Recently, we characterized TgCyp23 among the various Cyps of the parasite, demonstrating its high PPIase activity and its ability to bind cyclosporin A (CsA), a well‐known inhibitor of Cyps (Favretto et al., 2023). TgCyp23 exhibits the typical eight‐stranded antiparallel β‐barrel structure, with two α‐helices flanking the barrel on either side, all of them connected by loops. TgCyp23 shows remarkable sequence identity with human CypA (~52% of identity) but has a 40‐aminoacid N‐terminal extension. Here, three new structures of the protein in complex with the three non‐immunosuppressive derivatives NIM811, dhCsA, and Alisporivir have been solved at 1.17, 1.20, and 1.20 Å resolution, respectively.

Dihydrocyclosporin A (dhCsA), a closely related co‐metabolite of CsA, presents a saturation of the double bond of the unusual amino acid (4R)‐4‐([E]‐2‐butenyl)‐4‐methyl‐N‐methyl‐(L)‐threonine (MeBmt‐1) in position 1, has minimal reported immunosuppressive activity, and serves as a control in determining the role of immunosuppression in CsA‐based treatment of parasitic infections (Chappell et al., 1987; Meier et al., 1990). CsA derivatives with modifications at residue 1 (such as dhCsA, which is a co‐metabolite of CsA used as a control to determine the role of CsA in pharmacology) have also shown decreased immunosuppressive activity without compromising Cyp affinity, even though the MeBmt‐1 side chain is positioned in the part of CsA involved in the binding of Cyp (Aebi et al., 1990; Mikol et al., 1993; Rich et al., 1989). NIM811, dhCsA, and Alisporivir are attached to the CsA binding pocket. The backbone for these three derivatives is nearly identical to that of CsA. Remarkably, all the modifications in the non‐immunosuppressive derivatives are exposed, protrude from the binding site, and are not involved in the crystal packing. In all cases, the asymmetric unit is composed of two monomers with almost identical structure (RMSD values between 0.112 and 0.141 Å for the Cα superpositions). Remarkably, both NIM811 and dhCsA closely resembled the TgCyp23:CsA complex, implying that chemical modifications at position 4 of CsA exert negligible influence on the binding to the protein. Specifically, Alisporivir displayed the highest interaction affinity with TgCyp23 (Kd = 15 ± 3 nM) while dhCsA showed the lowest affinity (Kd = 200 ± 92 nM). The binding of all three compounds also had a significant impact on the thermal stability of the protein, leading to an overall increase in the melting temperature (Tm) of TgCyp23, as observed through both differential scanning calorimetry (DSC) and circular dichroism (CD) analysis. This effect consistently correlated with the higher binding affinity of Alisporivir and NIM811 to TgCyp23 compared to dhCsA, as determined by ITC analysis. All three compounds inhibit the catalytic activity of TgCyp23, with IC50 values between 0.8 and 2 nM, with Alisporivir having the highest inhibitory activity.

>GHMAPAPPANSGESSLLSESELPAGISYAEAMEGGSRPLLHPDNPVVFFDISIGSHEAGRIKIELFKNLAPKSAENFRQFCTGEFRQNQVPIGYKGATFHRIIKNFMIQGGDFVKGDGTGRLSIYGSSFPDEAFVLPHFRSGLLSLANSGPDTNGCQFFITCAKCDWLNRKHVVFGQVLGKESMQVVRKIEHVTVDGGNRPRIPVTVTQCGEL[2x];>[2x]ALLVTAGLVLA>GCGTAXACGC[2x]

Here, we report on incorporating an N-tert-butylguanidinium group at the 2′,4′-bridging structure, which greatly enhances duplex-forming ability because of its interactions with the minor groove. X-ray crystal structures of the self-complementary GuNA[Me,Me]- and GuNA[Me,tBu]-modified oligonucleotides showed that interactions between the N-tert-butyl group and the minor groove greatly enhanced the duplex stability. Two self-complementary sequences were selected; (1) a 10 mer oligodeoxynucleotide (5′-GCGTATACGC-3′)(35) and (2) an 8 mer oligodeoxynucleotide (5′-GTGBrUACAC-3′), where BrU represents a 5-bromourasil nucleobase(43)—these sequences have been used previously for crystallographic analysis. All three crystal structures were found to adopt the A-form duplex.

Among them, three oligonucleotides, ODN25, ODN28 and ODN29, formed good crystals for X-ray crystallographic analysis, and their crystal structures were successfully determined at the resolutions of 2.01, 0.95 and 0.93 Å, respectively. Intriguingly, two GuNA[Me,tBu]s in the duplexed ODN25 formed different structures from each other. The tert-butyl group of one was located at the minor groove side (see the GuNA[Me,tBu]-T6•dA15 base pair in Figure 3A, and C), whereas that of the other one was located outside of the duplex (see the GuNA[Me,tBu]-T16•dA5 base pair in Figure 3A and B). The results could be explained by a steric repulsion of the two tert-butyl groups because the GuNA[Me,tBu]s were located close together in the duplexed ODN25. This means that one of the tert-butyl groups at the minor groove exposed another tert-butyl group to the outside. On the other hand, two tert-butyl groups of the duplexed ODN29 were located on the minor groove side, and two GuNA[Me,tBu]s were found to have similar structures. Notably, we found that the tert-butyl-substituted guanidine moiety and the 2-carbonyl group of the thymine nucleobase formed a hydrogen bond (3.4 Å for ODN25 in Figure 3C and 3.2 Å for ODN29 in Figure 4B), suggesting that this additional hydrogen-bond contact, as well as the hydrophobic interactions between the tert-butyl group and the minor groove, contributed greatly to duplex stability. The extra hydrogen bond, observable in ODN25 and ODN28, would indirectly affect the strengths of the hydrogen bonds of base pairing and base stacking. Compared to the GuNA[Me,Me]-modified ODN24, GuNA[Me,tBu]-modified ODN25—in which one tert-butyl group flipped to the outside of the duplex—showed only a one-degree increase in the Tm value. In these three X-ray crystal structures, no counter anion was observed around the guanidium part.> SYHLDTTAPPPTNLSTLPNNTLFHLWRPRAHILPAEGQIGDPCAHYTDPSTGLFHVGFLHDGDGIAGATTANLATYTDTSDNGSFLIQPGGKNDPVAVFDGAVIPVGVNNTPTLLYTSVSFLPIHWSIPYTRGSETQSLAVARDGGRRFDKLDQGPVIADHPFAVDVTAFRDPFVFRSARLDVLLSLDEEVARNETAVQQAVDGWTEKNAPWYVAVSGGVHGVGPAQFLYRQNGGNASEFQYWEYLGEWWQEATNSSWGDEGTWAGRWGFNFETGNVLFLTEEGHDPQTGEVFVTLGTEGSGLPIVPQVSSIHDMLWAAGEVGVGSEQEGAKVEFSPSMAGFLDWGFSAYAAAGKVLPASSAVSKTSGVEVDRYVSFVWLTGDQYEQADGFPTAQQGWTGSLLLPRELKVQTVENVVDNELVREEGVSWVVGESDNQTATLRTLGITIARETKAALLANGSVTAEEDRTLQTAAVVPFAQSPSSKFFVLTAQLEFPASARSSPLQSGFEILASELERTAIYYQFSNESLVVDRSQTSAAAPTNPGLDSFTESGKLRLFDVIENGQEQVETLDLTV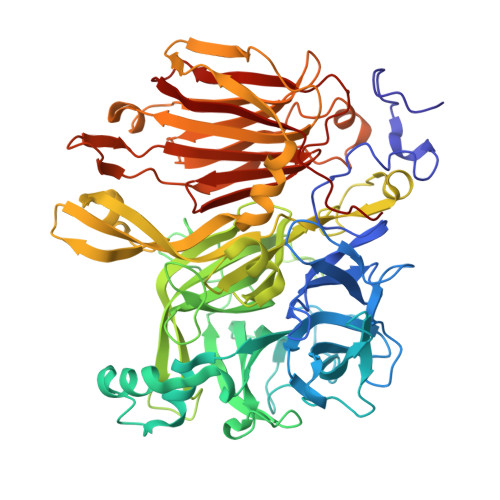VVDNAVVEVYANGRFALSTWARSWYDNSTQIRFFHNGEGEVQFRNVSVSEGLYNAWPER> 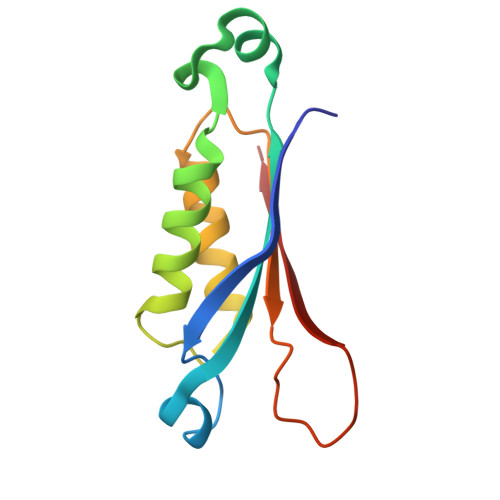MADRIELRGLTVHGRHGVYDHERVAGQRFVIDVTVWIDLAEAANSDDLADTYDYVRLASRAAEIVAGPPRKLIETVGAEIADHVMDDQRVHAVEVAVHKPQAPIPQTFDDVAVVIRRSR>[4x]MDWSHPQFEKSNRTPRRFRSRDWFDNPDHIDMTALYLERFMNYGITPEELRSGKPIIGIAQTGSDISPCNRIHLDLVQRVRDGIRDAGGIPMEFPVHPIFENCRRPTAALDRNLSYLGLVETLHGYPIDAVVLTTGCDKTTPAGIMAATTVNIPAIVLSGGPMLDGWHENELVGSGTVIWRSRRKLAAGEITEEEFIDRAASSAPSAGHCNTMGTASTMNAVAEALGLSLTGCAAIPAPYRERGQMAYKTGQRIVDLAYDDVKPLDILTKQAFENAIALVAAAGGSTNAQPHIVAMARHAGVEITADDWRAAYDIPLIVNMQPAGKYLGERFH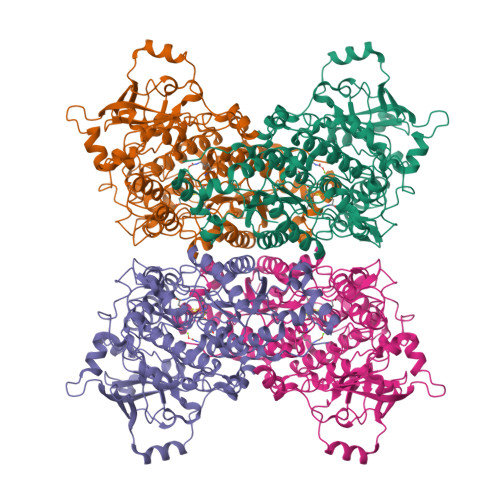RAGGAPAVLWELLQQGRLHGDVLTVTGKTMSENLQGRETSDREVIFPYHEPLAEKAGFLVLKGNLFDFAIMKSSVIGEEFRKRYLSQPGQEGVFEARAIVFDGSDDYHKRINDPALEIDERCILVIRGAGPIGWPGSAEVVNMQPPDHLLKKGIMSLPTLGDGRQSGTADSPSILNASPESAIGGGLSWLRTGDTIRIDLNTGRCDALVDEATIAARKQDGIPAVPATMTPWQEIYRAHASQLDTGGVLEFAVKYQDLAAKLPRHNH>[2x]MAVPTGSANLFLRPLILAVLSFLLLSSFVSSVEWLDIDSSDLKALQVIETELGVNSQRS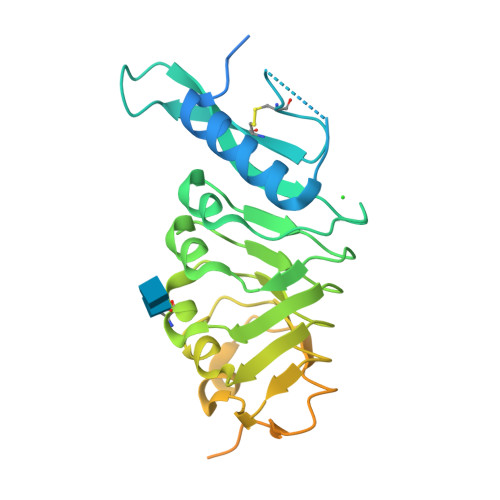SASDVNPCGRRGVFCERRHSATTGEYVLRVTRLVYRSRSLTGTISPVIGMLSELKELTLSNNQLVNAVPVDILSCKQLEVLDLRKNRFSGQIPGNFSSLSRLRILDLSSNKLSGNLNFLKNLRNLENLSVANNLFSGKIPEQIVSFHNLRFFDFSGNRYLEGPAPVMSSIKLQTSPHQTRHILAETPTSSPTNKPNNSTTSKAPKGAPKPGLELENLYFQGAWSHPQFEKGSHHHHHHHHH>MNQNLLVTKRDGSTERINLDKIHRVLDWAAEGLHNVSISQVELRSHIQFYDGIKTSDIHETIIKAAADLISRDAPDYQYLAARLAIFHLRKKAYGQFEPPALYDHVVKMVEMGKYDNHLLEDYTEEEFKQMDTFIDHDRDMTFSYAAVKQLEGKYLVQNRVTGEIYESAQFLYILVAACLFSNYPRETRLQYVKRFYDAVSTFKISLPTPIMSGVRTPTRQFSSCVLIECGDSLDSINATSSAIVKYVSQRAGIGINAGRIRALGSPIRGGEAFHTGCIPFYKHFQTAVKSCSQGGVRGGAATLFYPMWHLEVESLL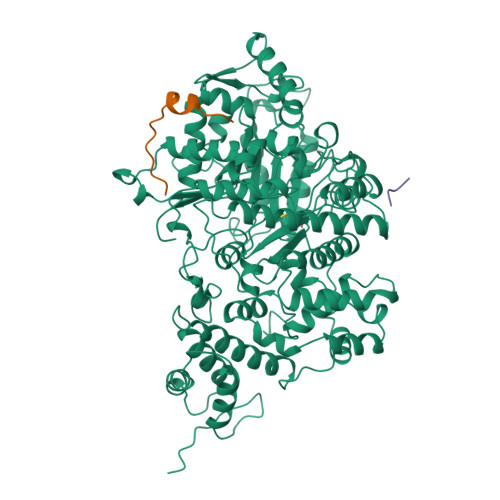VLKNNRGVEGNRVRHMDYGVQINKLMYTRLLKGEDITLFSPSDVPGLYDAFFADQEEFERLYTKYEKDDSIRKQRVKAVELFSLMMQERASTGRIYIQNVDHCNTHSPFDPAIAPVRQSNLCLAIALPTKPLNDVNDENGEIALCTLSAFNLGAINNLDELEELAILAVRALDALLDYQDYPIPAAKRGAMGRRTLGIGVINFAYYLAKHGKRYSDGSANNLTHKTFEAIQYYLLKASNELAKEQGACPWFNETTYAKGILPIDTYKKDLDTIANEPLHYDWEALRESIKTHGLRNSTLSALMPSETSSQISNATNGIEPPRGYVSIKASKDGILRQVVPDYEHLHDAYELLWEMPGNDGYLQLVGIMQKFIDQSISANTNYDPSRFPSGKVPMQQLLKDLLTAYKFGVKTLYYQNTRDGAEDAQDDLVPSIQDDGCESGACKI[3x];>[4x]YLVGQIDSEVDTDDLSNFQL>[2x]NU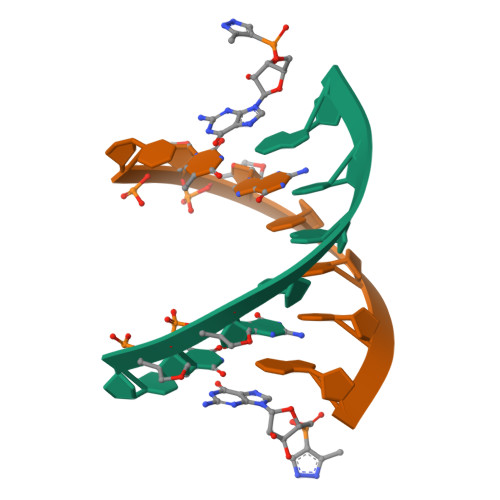GUACA MpPA14 (Marinomonas primoryensis PA14 domain) lectin is a domain of a 1.5-MDa adhesin responsible for a symbiotic bacterium-diatom interaction in Antarctica. Bioinformatic analyses indicated the presence of an ∼20-kDa domain near the C terminus of MpIBP that is a member of the PA14 family, which is a carbohydrate-binding lectin module widely distributed across several kingdoms of life. PA14 domains share a β-sandwich fold and the presence of two consecutive aspartate residues in a cis peptide linkage (DcisD). The DcisD motif coordinates a Ca2+ ion that is directly involved in binding polar vicinal hydroxyl groups of various carbohydrates.

Galactose has its C-4 hydroxyl in the axial position instead of being equatorial as in glucose. Docking of the galactopyranose ring to MpPA14 via the 3,4-diol is not possible due to steric hinderance against Gln129 and Ser130 on L-9. Instead, galactose can only interact with MpPA14 via the 1,2-diol of its rare β-anomer. These limitations explain the relatively weak interaction between galactose and MpPA14. Having just shown the 3,4-diol of galactopyranose cannot complex MpPA14, binding of GalNAc is completely abolished because its 1,2-diol is unavailable due to the C-2 hydroxyl being substituted with an acetyl group. Similarly, since the MpPA14 binds galactose via the 1,2-diol (β-anomer), the lectin cannot interact with galactans, as they are polymers of β-1,4-d-galactose.

> KAQDDSTPDSLFAGLVGEYYGTNSQLNNISDFRALVDSKEADATFEAANISYGRGSSDVAKGTHLQEFLGSDASTLSTDPGDNTDGGIYLQGYVYLEAGTYNFKVTADDGYEITINGNPVATVDNNQSVYTVTHASFTISESGYQAIDMIWWDQGGDYVFQPTLSADGGSTYFVLDSAILSSTGETPY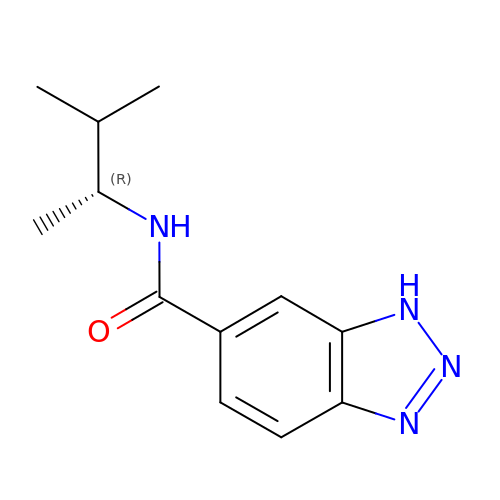N-[(2R)-3-methylbutan-2-yl]-1H-benzotriazole-6-carboxamide | C12 H16 N4 O | ONKYUGFAMPVNLE-MRVPVSSYSA-N> MWPSARFVDDNVAFSRMPTERELDEVAKDFDAVVVLVEEYELPYSLEEWKKRGVEVLHSPIPDFTAPSLEQLLEILRWIEARVREGKKVLIHCMGGLGRSGTVAVAWLMYSKGLPLREALR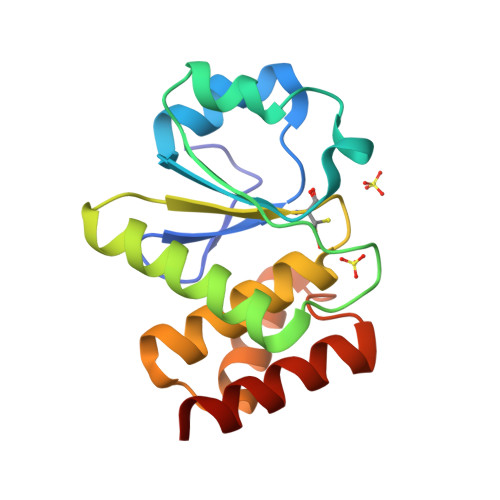RVRSLRPGAVETYEQMEVLKELEKFLRSR>[4x]KAVPQCEPGSGFSFELTEQQKEFQATARKFAREEIIPVAAEYDRTGEYPVPLLKRAWELGLMNTHIPESFGGLGLGIIDSCLITEELAYGCTGVQTAIEANTLGQVPLIIGGNYQQQKKYLGRMTEEPLMCAYCVTEPGAGSDVAGIKTKAEKKGDEYIINGQKMWITNGGKANWYFLLARSDPDPKAPASKAFTGFI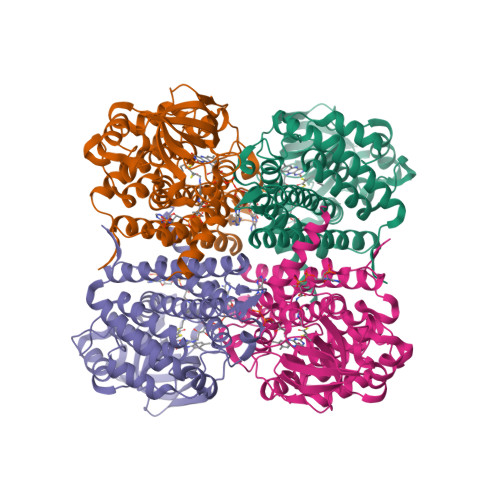VEADTPGVQIGRKEINMGQRCSDTRGIVFEDVRVPKENVLTGEGAGFKIAMGTFDKTRPPVAAGAVGLAQRALDEATKYALERKTFGKLLAEHQGISFLLADMAMKVELARLSYQRAAWEIDSGRRNTYYASIAKAYAADIANQLATDAVQVFGGNGFNTEYPVEKLMRDAKIYQIYEGTAQIQRIIIAREHIGRYKN>[18x]MASTATVATTPEGIPVIILKEGSSRTYGKEAVRANIAAVKA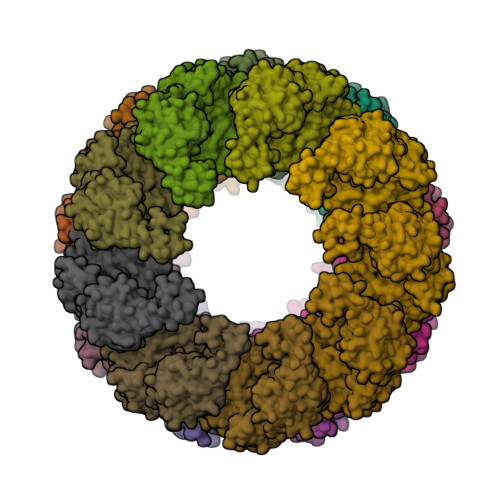VEEALKSTYGPRGMDKMLVDSLGDITITNDGATILDKMDLQHPAAKLLVQIAKGQDEETADGTKTAVIFSGELVKKAEDLLYKDVHPTIIISGYKKAEEVALQTIQELAQTVSINDTDLLRKIAMTSLSSKAVAGAREYIADIVVKAVTQVAELRGDKWYVDLDNIQIVKKAGGSINDTQLVYGIVVDKEVVHPGMPKRLENAKIALIDASLEVEKPELDAEIRINDPTQMQKFLDEEENLIKEKVDKILATGANVIICQKGIDEVAQSYLAKKGVLAVRRAKKSDLEKLARATGGRVVSNIDEISEQDLGYASLIEERKVGEDKMVFVEGAKNPKSISILIRGGLERLVDETERALRDALGTVADVIKDGRAIAGGGAVEIEIAKKLRKYAPQVGGKEQLAVEAYANALESLVSILIENAGFDPIDLLMKLRSTHENENNKWYGIDLYAGQPVDMWQKGVIEPALVKMNAIKAATEAATLVLRIDDVVSAGKKSGGESKTPGGANKPSEED> ESYCGPCPKNWICYKNNCYQFFDESKNWYESQASCMSQNASLLKVYSKEDQDLLKLVKSYHWMGLVHIPTNGSWQWEDGSILSPNLLTIIEMQKGDCALYASSFKG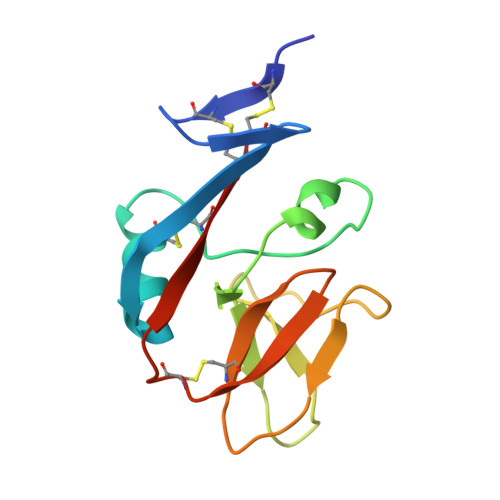YIENCSTPNTYICMQRTV>AYPMPNPFPPFRIAGNLYYVGTDDLASYLIVTPR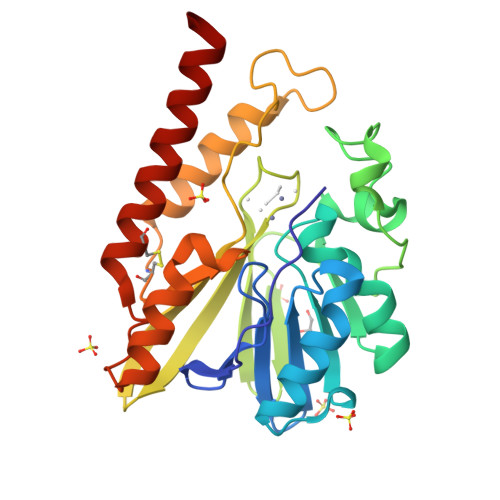GNILINSDLEANVPMIKASIKKLGFKFSDTKILLISHAHFDHAAGSELIKQQTKAKYMVMDEDVSVILSGGKSDFHYANDSSTYFTQSTVDKVLHDGERVELGGTVLTAHLTPGHTRGCTTWTMKLKDHGKQYQAVIIGSIGVNPGYKLVDNITYPKIAEDYKHSIKVLESMRCDIFLGSHAGMFDLKNKYVLLSKGQNNPFVDPTGCKNYIEQKANDFYTELKKQETG[2x]> MRVKVIDADAFSYIFRTLEEFIDEITLDFTSDGLKIRGIDPSRVTFIDILIPAGYFEEYNVEKEEKVGVKLEDFTDVLKTVTKNDSLYLETDENQNIKVTLDGVYERTFTFPSIVASEIETPNLNLEFPFKAKALTVTFTDIIDEIEDIGGDSITFKAEGGKLYLSANSDMGSSTIELSTENGGLLESEGGDAESVYGLEYVVNTSKMRKPSDTVEIAFGSQIPLKLRYNLPQGGYADFYIAPRAE;> MIKATYSSAKDFYSLLSGLLKVTDEIILNFTEDSIFSRYLTDDKVLMVIFKIPKEYLEDYTIDK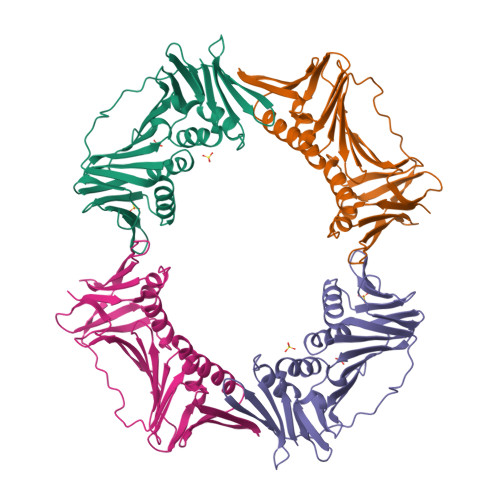PLGIKININDLKKILGKAKSKSATVTLEETEAGLKVTVRDEKTGTRSNIYIKGEKTSIDQLTEPKVNLSVTFTTDGDVLKDIARDLSLVGEEVEISADENTVTLSTEEAGRTYKSLLKQDKPLKSLNVESPSKAVYSIEVLKDVFKVTSISQNVTVGFGNNIPMKIEVPTDSGGQLIFWIAPRL>MHHHHHHSAGENLYFQGKEWQENKSWNAHFTEHKSQGVVVLWNENKQQGFTNN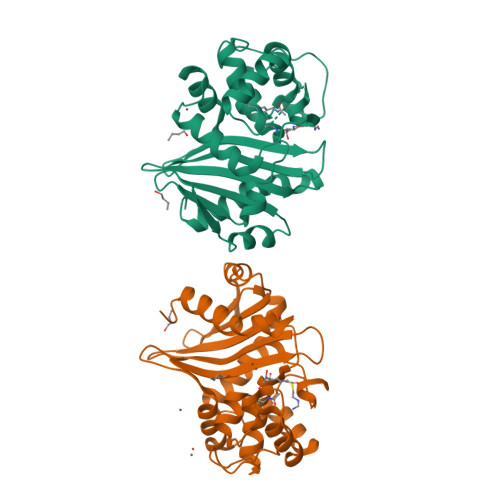LKRANQAFLPASTFKIPNSLIALDLGVVKDEHQVFKWDGQTRDIATWNRDHNLITAMKYSVVPVYQEFARQIGEARMSKMLHAFDYGNEDISGNVDSFWLDGGIRISATEQISFLRKLYHNKLHVSERSQRIVKQAMLTEANGDYIIRAKTGYSTRIEPKIGWWVGWVELDDNVWFFAMNMDMPTSDGLGLRQAITKEVLKQEKIIP[8x]> SNATGERFHPLLGRRVPDPAPGARCFTGTVSSDRPAYLGEHWVYDAIVVLGVTYLEMALAAASRLLPGNAADTLIVEDVTVWSPLVLRAGAPARLRLRSEDERFEIHSAEPERSDDESAWTRHATGRIARRQLSPDATGQLPRLDGEAVELDAYYERMRIYY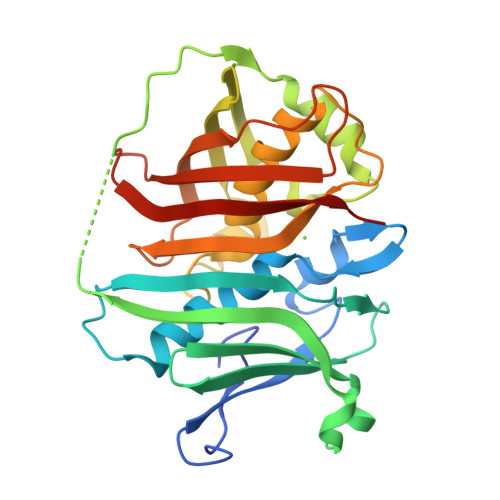GPRLRNIRHLERRGREAIGHVCLQGEEAQESASYELHPALLDACFQCVFALIYAHESHREPFVPLGCARIELRARGVREVRVHLRLHPPRSTDHNQTHTADLRLFDMEGRLVASVDALQLKRASKAALL> MHHHHHHITSLYKKAGSEFALDSSKLEAIYATSEADRDYKENAVDGDENTIWHSAYQAADKLPVSITIKLDKAYDLNQIDYLPRQNSRNGHVTEYKIETSLDNENWTEVRTGNLEVNEAGNALANRGYNPIRFNTINAQYLRFTALKTLGDTNNKYASAAELVFYGK

As part of the secreted C. perfringens CAZyme arsenal, the bacterium possesses an open reading frame coding for a 220-kDa family 31 glycoside hydrolase (locus tag CPF_1301 in strain ATCC 13124) with predicted α-glucosidase activity, which will be hereafter referred to as CpGH31. In addition to the N-terminal glycoside hydrolase family 31 catalytic module, CpGH31 comprises two fibronectin-type III modules, three CBM32s, a putative cohesin module, and a bacterial immunoglobulin-like 2 module. Though the putative CBMs, referred to as CBM32-1, CBM32-2, CBM32-3, themselves are not closely related at the amino acid sequence level, a primary structure comparison indicates that they all belong to CBM family 32, an observation that is supported by their overall similar structures as determined by X-ray crystallography. Each CpGH31 CBM32 structure comprised the β-sandwich topology characteristic of this CBM family with a short α-helix and a calcium ion capping one side of each module.

The molecular determinants of galacto-specific sugar recognition displayed by CpGH31 CBM32-3 were revealed by the X-ray crystal structures of this protein module in its apo-, galactose-bound, and GalNAc-bound states, which were determined to 1.58 Å, 1.48 Å and 2.50 Å resolution, respectively. The galactose and GalNAc residues were well-ordered in the crystal structures of the CBM32-3:Gal and CBM32-3:GalNAc complexes, respectively, and provided clear electron density, allowing for monosaccharide modeling into each structure. The galactose and GalNAc coordinating amino acid residues of CBM32-3 were conserved, and included Tyr1674, His1671, Arg1702, Asn1707 and Tyr1774. The b-face of both sugars formed CH-π interactions with Tyr1674, while a secondary aromatic residue, Tyr1774, whose side chain is perpendicular to that of Tyr1674, mediated additional hydrophobic interactions with the C6 group of each sugar. Galactose and GalNAc binding was further stabilized through a series of polar contacts formed between the side chains of His1671, Arg1702 and Asn1707 and the C2-C3-C4-C5 edge of each sugar. Specifically, hydrogen bonds were observed between Asn1707 and the O4 hydroxyl and endocyclic oxygen, His1671 and the O4 hydroxyl, and Arg1702 and the O3 and O4 hydroxyl and 2-acetamido groups. The orientation of galactose and GalNAc, and the respective contacts being made with the CBM were consistent with the STD NMR data, in which strong STD signals for the apolar α- and β-H3, α- and β-H4, α/β-H6, and acetyl group protons were observed. Alignment of the three CBM32-3 structures revealed minimal sugar—induced structural changes (backbone r.m.s.d < 0.22 Å) and only subtle differences in B-factors associated with the variable loops were also observed.D-Xylose, 4-O-beta-D-xylopyranosyl- | C10 H18 O9 | 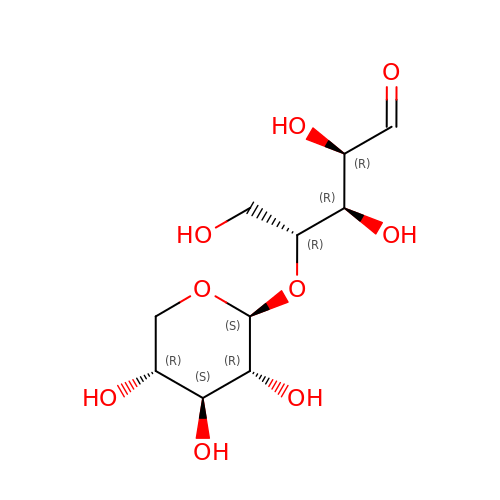SQNRKWHRVIAKLP-RSZZQXBVSA-N>NNKTLAAMKNFAEQYAKRTDT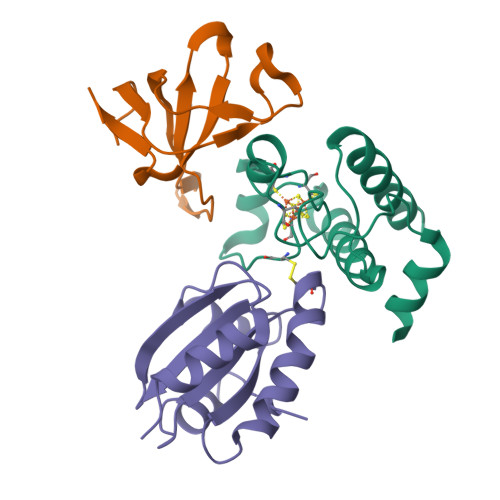YFCSDLSVTAVVIEGLARHKEELGSPLCPCRHYEDKEAEVKNTFWNCPCVPMRERKECHCMLFLTPDNDFAGDAQDIPMETLEEVKAS[2x];>[2x]MNVGDRVRVTSSVVVYHHPEHKKTAFDLQGMEGEVAAVLTEWQGRPISANLPVLVKFEQRFKAHFRPDEVTLI;>[2x]EVQDVNDSSWKEFVLESEVPVMVDFWAPWCGPSKLIAPVIDELAKEYSGKIAVYKLNTDEAPGIATQYNIRSIPTVLFFKNGERKESIIGAVPKSTLTDSIEKYLS> MNIRLHGLTTILSALVVLTAPTAVLAQDNLVTGELITTVNSGTPGKGGEVTFAVTRDITNWNVTSALGNNAVVRTVTLPIVPSAFMVQPDF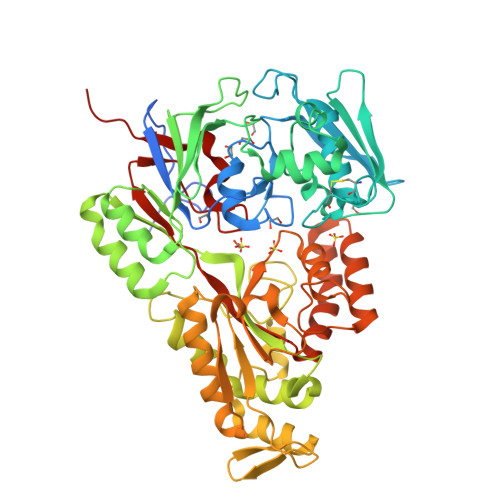TLKMNTDLLESAELTSTDPQTVVYRIREDAVWSDGVPITGDDFIYFWKTQNRRDCPECLINASYGHDFIETLEQDETGKVVTATFSEPFLGWQGLFMFLYPAHLAEKHGDIAESYNNFLSNEVPAWSGGPYMVESFDPGQLVTLVPNPKWYGEKGPYLDKLKFRIITDSTQQLTALENGEVDVIYPQGATQDMVEQAAGLDYLGIDFQMNPSANWYFMGLNSKAGPMSDIALRKAVLTAIDAGDLKAKTADPYLRNWPHMGSVMFLPNQAGYADRRGARGYGTGDVEKAKGILSEAGYKLSGGSLLDPSGKPVSTLRLSFPPGYPAANDMARLITGYIAPLGLKTDLLTGPNATADYLLSGNFDLHLNYFSQQVFPAVKAGQIFLRDTRQNYFGFNDPKIEEIIGKAAAASSIEESAAILSEADELAMDYAALFPIYQLPTALIYKEAILNLRDNPNQLGPAYNTAEWGLAELEHHHHHH> Q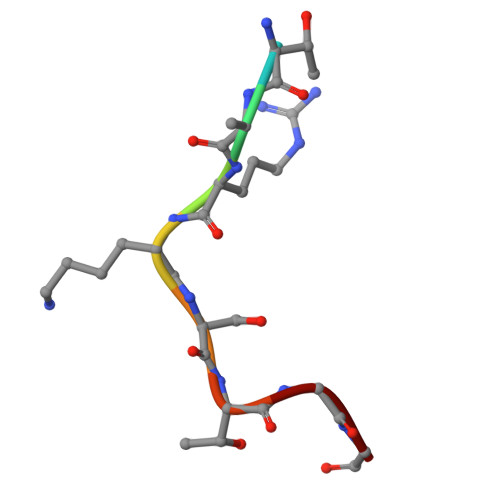TARKSTGG>[4x]MHIERLAVDESVGRAMPPQRFIEALSDLGVPVEFAGEDEQFGPGD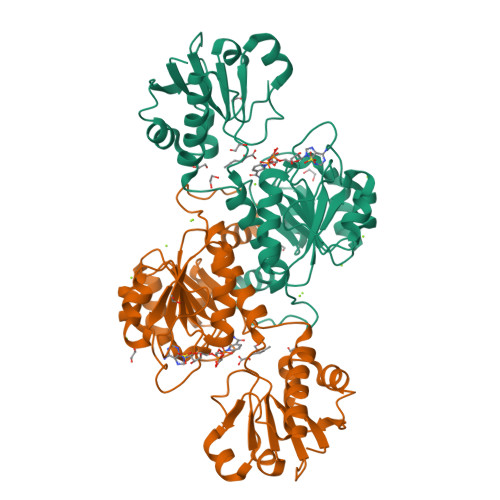AVASFGHRDAFLDADWVHCIRAGYDEFPVGVYEEAGTYLTNSTGIHGTTVGETVAGYMLTFARRLHAYRDAQHDHAWDLPRYEEPFTLAGERVCVVGLGTLGRGVVDRAAALGMEVVGVRRSGDPVDNVSTVYTPDRLHEAIADARFVVLATPLTDETEGMVAAPEFETMREDASLVNVARGPVVVESDLVAALDSGDIAGAALDVFSEEPLPEDSPLWDFEDVLITPHVSAATSKYHEDVAALIRENIEKIATGDELTNRVV>LLSPETIEALRKPTFDVWLWEPNEMLSCLEHMYHDLGLVRDFSINPVTLRRWLFCVHDNYRNNPFHNFRHCFCVAQMMYSMVWLCSLQEKFSQTDILILMTAAICHDLDHPGYNNTYQINARTELAVRYNDISPLENHHCAVAFQILAEPECNIFSNIPPDGFKQIRQGMITLILATDMARHAEIMDSFKEKMENFDYSNEEHMTLLKMILIKCCDISNEVRPMEVAEPWVDCLLEEYFMQSDREKSEGLPVAPFMDRDKVTKATAQIGFIKFVLIPMFETVTKLFPMVEEIMLQPLWESRDRYEELKRIDDAMK[2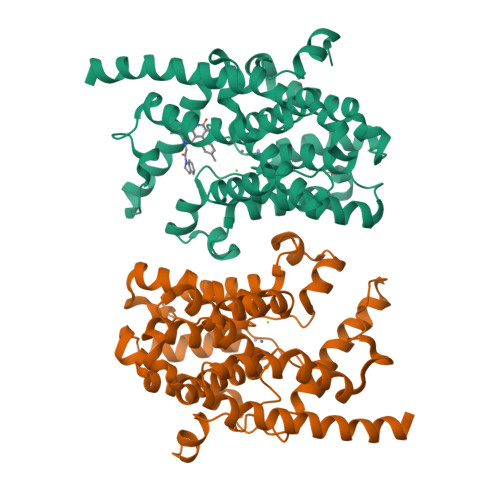x]> QAIKESYAFAVLGEPRYAFNFNHFDYVNPAAPKGGQITLSALGTFDNFNRYALRGNPGARTEQLYDTLFTTSDDEPGSYYPLIAESARYADDYSWVEVAINPRARFHDGSPITARDVEFTFQKFMTEGVPQFRLVYKGTTVKAIAPLTVRIELAKPGKEDMLSLFSLPVFPEKYWKDHKLSDPLATPPLASGPYRVTSWKMGQNIVYSRVKDYWAANLPVNRGRWNFDTIRYDYYLDDNVAFEAFKAGAFDLRMENDAKNWATRYTGKNFDKKYIIKDEQKNESAQDTRWLAFNIQRPVFSDRRVREAITLAFDFEWMNKALFYNAWSRTNSYFQNT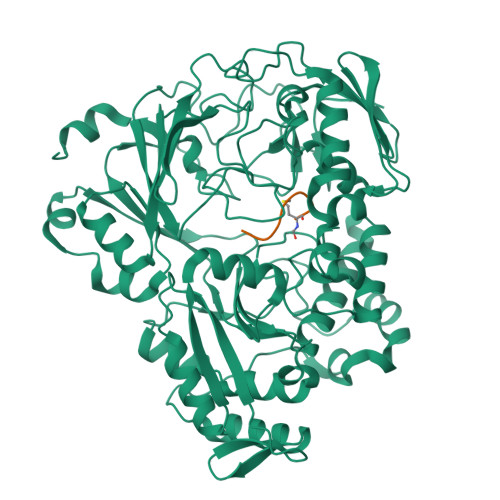EYAARNYPDAAELVLLAPMKKDLPSEVFTQIYQPPVSKGDGYDRDNLLKADKLLNEAGWVLKGQQRVNATTGQPLSFELLLPASSNSQWVLPFQHSLQRLGINMDIRKVDNSQITNRMRSRDYDMMPRVWRAMPWPSSDLQISWSSEYINSTYNAPGVQSPVIDSLINQIIAAQGNKEKLLPLGRALDRVLTWNYYMLPMWYMAEDRLAWWDKFSQPAVRPVYSLGIDTWWYDVNKAAKLPSASKQGE;> MRTGNAN>MKNVLVFLILLVALPALAQGHKPLEVIKIEDGVYLHTSFKNIEGYGLVDSNGLVVLDNNQAYIIDTPWSEEDTKLLLSWATDRGYQVMASISTHSHEDRTAGIKLLNSKSIPTYTSELTKKLLAREGKPVPTHYF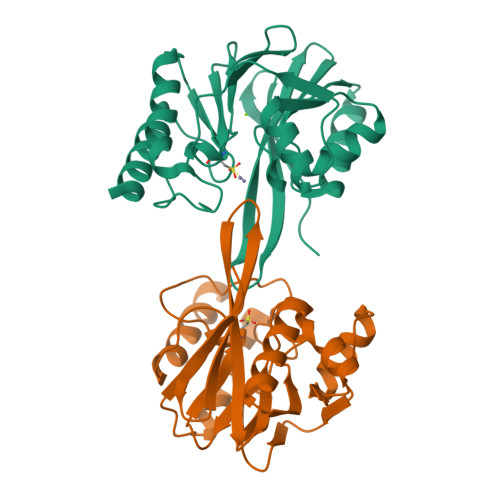KDDEFTLGNGLIELYYPGAGHTEDNIVAWLPKSKILFGGCLVRSHEREGLGYVGDASISSWADSIKNIVSKKYPIQMVVPGHGKVGSSDILDHTIDLAESASNKLMQPTAEASAD[2x]>MLMRATLTVLGSGTSMGVPTIGCDCAVCSSSDPHDRRLRPSVMVQYDGKLVLIDTTPDFREQALREGIKKIDAIVYTHGHADHILGLDDVRPLSFPRITGGARVPLYANEK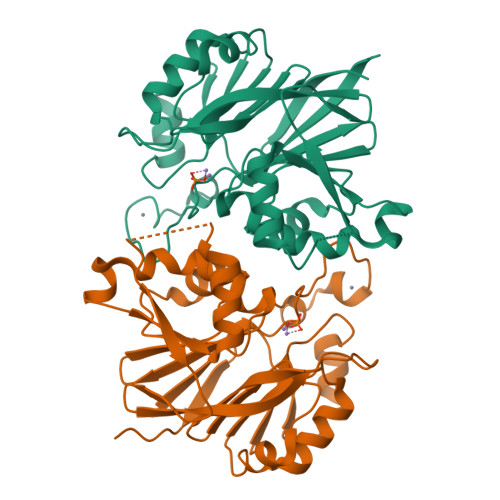TERVLKHVFKYIFDDDYKFGSIAQVEMHRVHHEAIELFGAKFIPVPVIHGETEIYGYRFGSAAYLTDFSSIPDASMEMLRGLDILFLDALRHKPHPTHSTLDNSVSIAEKLKAKHTYFTHISHDLPHEETNRQLPAGIQLAHDGLKLEFELCLEHHHHHH[2x]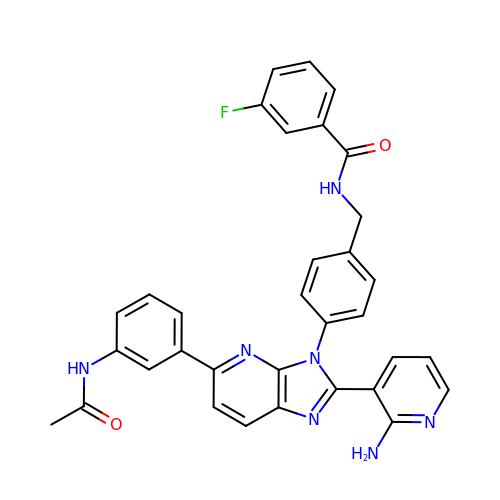N-(4-{5-[3-(acetylamino)phenyl]-2-(2-aminopyridin-3-yl)-3H-imidazo[4,5-b]pyridin-3-yl}benzyl)-3-fluorobenzamide | C33 H26 F N7 O2 | WFDHLKUQFQCHKF-UHFFFAOYSA-N>[2x]DEPVTY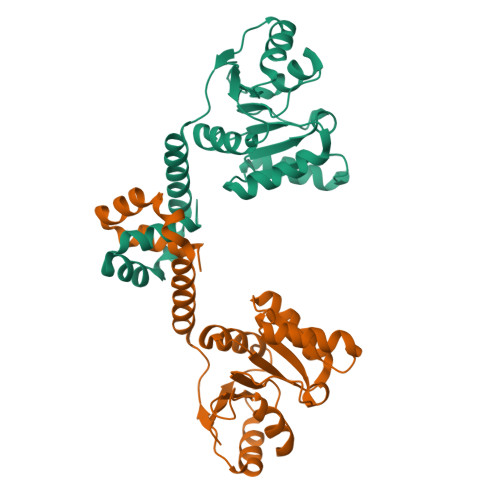EEEAVPAPVRGRLEVLSDLLYVASPDRAMVFTRTKAETEEIAQGLLRLGHPAQALHGDLSQGERERVLGAFRQGEVRVLVATDVAARGLDIPQVDLVVHYRLPDRAEAYQHRSGRTGRAGRGGRVVLLYGPRERRDVEALERAVGRRFKRVNPPTPEEVLEAKWRHLLARLARVPEKDYRLYQDFAGRLFAEGRVEVVAALLALLL>GSGNSHTTPWTNPGLAENFMNSFMQGLSSMPGFTASQLDNMSTIAQSMVQSIQSLAAQGRTSPNKLQALNMAFASSMAEIAASQEGGGSLSTKTSSIASAMSNAFLQTTGV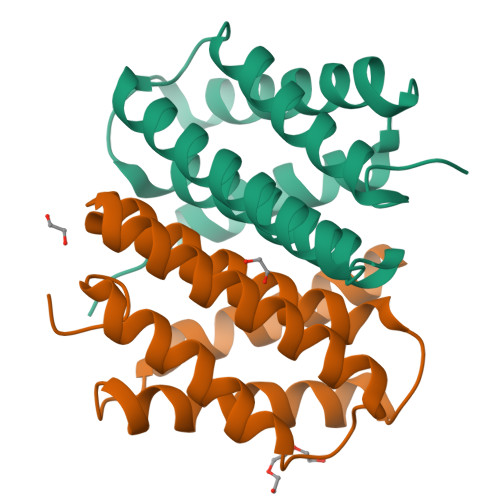VNQPFINEITQLVSMFAQAGMNDVSA[2x]>[3x]GMKVTFLGHAVVLIEGKKNIIIDPFISGNPVCPVKLEGLPKIDYILVTHGHGDHLGDAVEIAKKNDATVISNYEICHYLG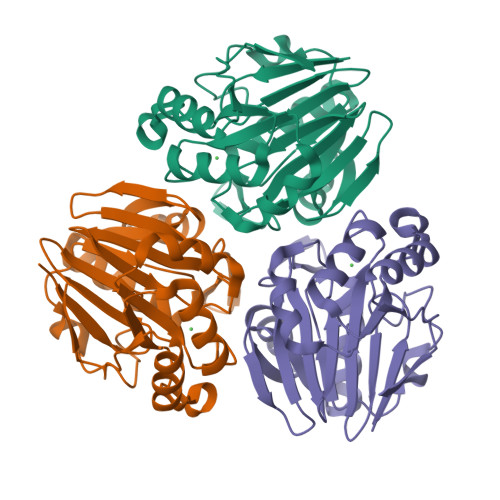KKGVKTHAMHIGGSYLFDFGRVKMTPAVHGSGILDGDSMIYGGNPSGFLITIEGKKIYHAGDTGLTREMELLAEENVDVAFLPIGGNFVMDVEDAVRAAVMIKPKKVVPMHYGTWELIFADVELFKKKVEEKGVECVILEPGESLEL>MASTAAETEKPEDHNDLVQLCNPHIAAMKEDILYHFSLSTSTHDFPAMFGDVKFVCVGGSPSRMKAFIKYVAMELGFAHPGADYPNICEGTDRYAMFKVGPVLSVSHGMGVPSIAIMLHELIKLLYHAHCSGVTLIRIGTSGGIGLEPGSVVITRQAVDPCFKPEFEQIVLGKREVRNTDLDEQLVQELARCSAELGEFPTVVGNTMCTLDFYEGQGRLDGALCSYTEKDKQDYLRAAYAAGIRNIEMEASVFAAMCNACGLRAAVVCVTLLNRLEGDQISSPHDVLAEYQQR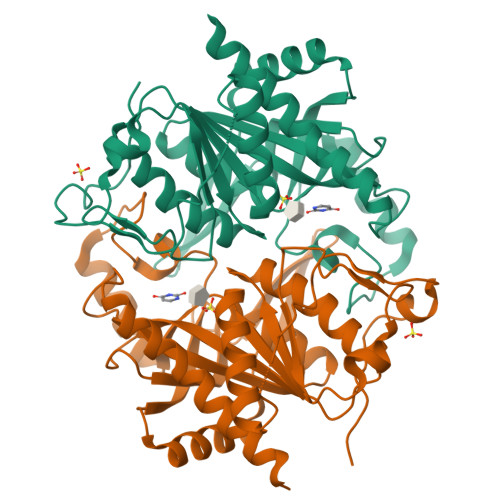PQRLVGQFIKKRLMQA[2x]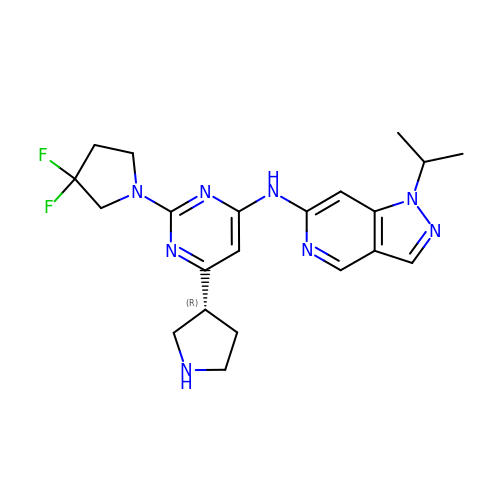N-{2-(3,3-difluoropyrrolidin-1-yl)-6-[(3R)-pyrrolidin-3-yl]pyrimidin-4-yl}-1-(propan-2-yl)-1H-pyrazolo[4,3-c]pyridin-6-amine | C21 H26 F2 N8 | JKPAJCPZQIJPPS-CQSZACIVSA-N> MARRILVVEDEAPIREMVCFVLEQNGFQPVEAEDYDSAVNQLNEPWPDLILLAWMLPGGSGIQFIKHLK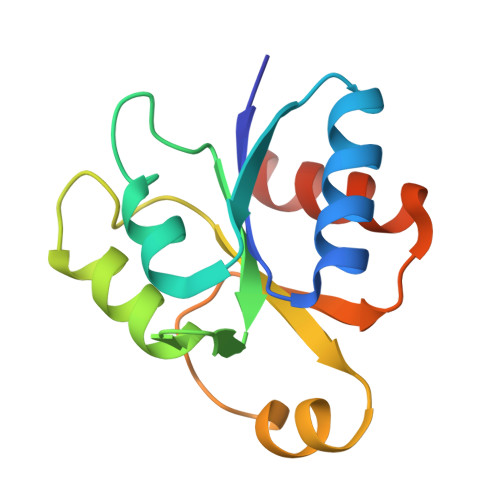RESMTRDIPVVMLTARGEEEDRVRGLETGADDCITKPFSPKELVARIKAVMRRISPMA> GVVPQYGGGGNHGGGGNNSGP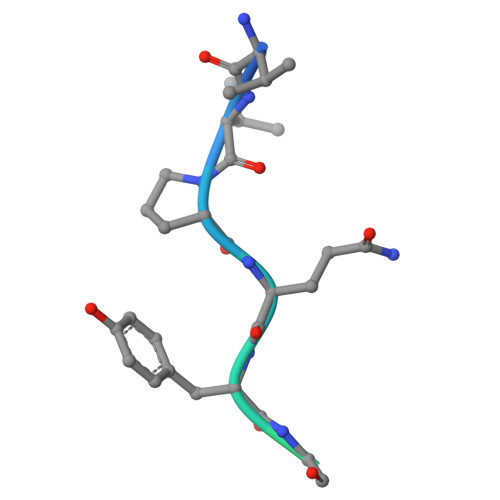N>[2x]MSSKEQKTPEGQAPEEIIMDQHEEIEAVEPEASAEQVDPRDEKVANLEAQLAEAQTRERDGILRVKAEMENLRRRTELDIEKAHKFALEKFINELLPVIDSLDRALEVADKANPDMSAMVEDIELTLKSMLDVVRKFGVEVIAETNVPLDPNVHQAIAMVESDDVAPGNVLGIMQKGYTLNGRTIRAAMVTVAKAKA;> MGKI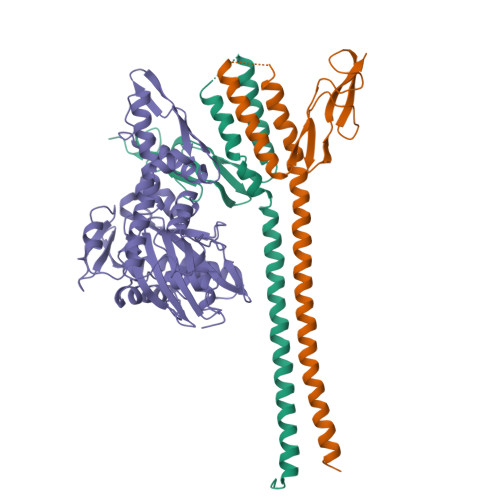IGIDLGTTNSCVAIMDGTTPRVLENAEGDRTTPSIIAYTQDGETLVGQPAKRQAVTNPQNTLFAIKRLIGRRFQDEEVQRDVSIMPFKIIAADNGDAWVEVKGQKMAPPQISAEVLKKMKKTAEDYLGEPVTEAVITVPAYFNDAQRQATKDAGRIAGLEVKRIINEPTAAALAYGLDKGTGNRTIAVYDLGGGTFDISIIEIDEVDGEKTFEVLATNGDTHLGGEDFDSRLINYLVEEFKKDQGIDLRNDPLAMQRLKEAAEKAKIELSSAQQTDVNLPYITADATGPKHMNIKVTRAKLESLVEDLVNRSIELLKVALQDAGLSVSDIDDVILVGGQTRMPMVQKKVAEFFGKEPRKDVNPDEAVAIGAAVQGGVLT>MKTVTVKNLIIGEGMPKIIVSLMGRDINSVKAEALAYREATFDILEWRVDHFMDIASTQSVLTAARVIRDAMPDIPLLFTFRSAKEGGEQTITTQHYLTLNRAAIDSGLVDMIDLELFTGDADVKATVDYAHAHNVYVVMSNHD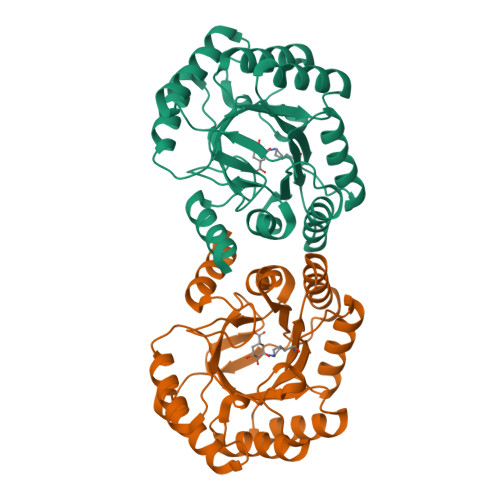FHQTPSAEEMVLRLRKMQALGADIPKIAVMPQSKHDVLTLLTATLEMQQHYADRPVITMSMAKEGVISRLAGEVFGSAATFGAVKQASAPGQIAVNDLRSVLMILHNA[2x]> 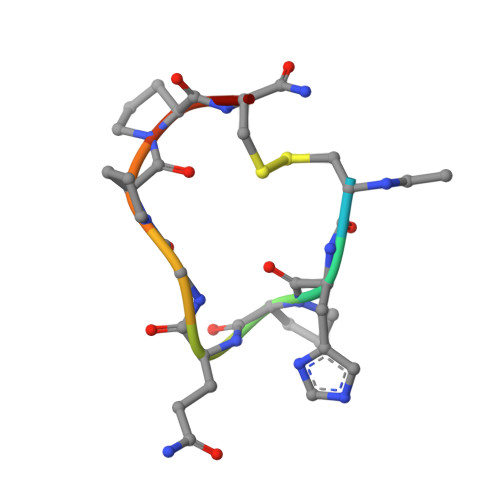XCHPQGPPCX>MPLGLLWLGLALLGALHAQAQDSTSDLIPAPPLSKVPLQQNFQDNQFQGKWYVVGLAGNAILREDKDPQKMYATIYELKEDKSYNVTSVLFRKKKCDYWIRTFVPGSQPGEFTLGNIKSYPG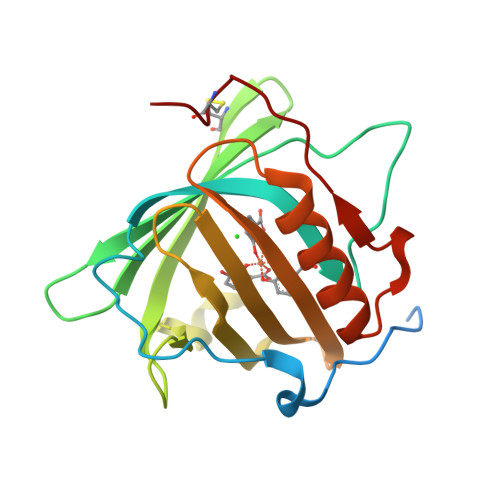LTSYLVRVVSTNYNQHAMVFFKKVSQNREYFKITLYGRTKELTSELKENFIRFSKSLGLPENHIVFPVPIDQCIDG[4x]> HGTELPSPPSVWFEAEFFHHILHWTPIPQQSESTCYEVALLRYGIESWNSISQCSQTLSYDLTAVTLDLYHSNGYRARVRAVDGSRHSQWTVTNTRFSVDEVTLTVG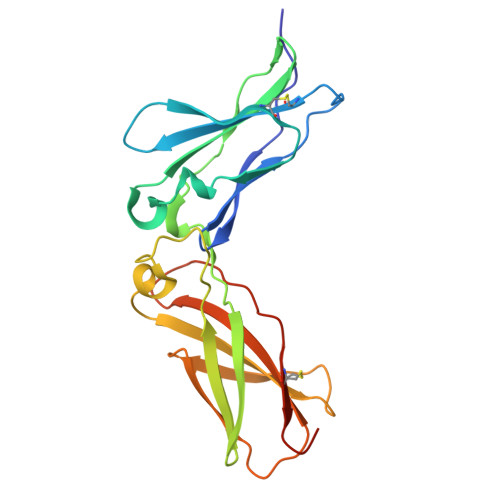SVNLEIHNGFILGKIQLPRPKMAPAQDTYESIFSHFREYEIAIRKVPGQFTFTHKKVKHEQFSLLTSGEVGEFCVQVKPSVASRSNKGMWSKEECISLTRQYFTVTN>[4x]VPRGSPWFGMDIGGTLVKLSYFEPIDITAEEEQEEVESLKSIRKYLTSNVAYGSTGIRDVHLELKDLTLFGRRGNLH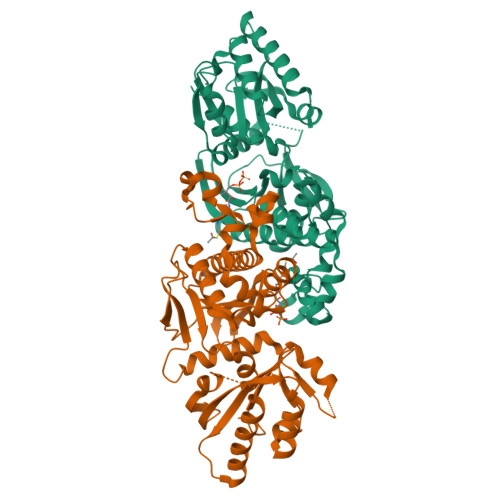FIRFPTQDLPTFIQMGRDKNFSTLQTVLCATGGGAYKFEKDFRTIGNLHLHKLDELDCLVKGLLYIDSVSFNGQAECYYFANASEPERCQKMPFNLDDPYPLLVVNIGSGVSILAVHSKDNYKRVTGTSLGGGTFLGLCSLLTGCESFEEALEMASKGDSTQADKLVRDIYGGDYERFGLPGWAVASSFGNMIYKEKRESVSKEDLARATLVTITNNIGSVARMCAVNEKINRVVFVGNFLRVNTLSMKLLAYALDYWSKGQLKALFLEHEGYFGAVGALLGLPN(2S)-2-[[(2S)-2-[2-[(2-azanyl-4-oxidanylidene-1H-pteridin-7-yl)carbonylamino]ethanoylamino]-3-phenyl-propanoyl]amino]-3-phenyl-propanoic acid | C27 H26 N8 O6 | 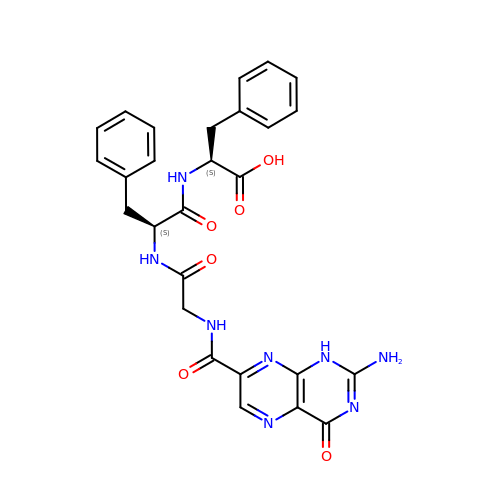ANWDLDKKFUMOHP-ROUUACIJSA-N>GGEERLETPSAKKLTDIGIRRIFSPEHDIFRKSVRKFFQEEVIPHHSEWEKAGEVSREVWEKAGKQGLLGVNIAEHLGGIGGDLYSAAIVWEEQAYSNCSGPGFSIHSGIVMSYITNHGSEEQIKHFIPQMTAGKCIGAIAMTEPGAGSDLQGIKTNAKKDGSDWILNGSKVFISNGSLSDVVIVVAVTNHEAPSPAHGISLFLVENGMKGFIKGRKLHKMGLKAQDTAELFFEDIRLPASALLGEENKGFYYIMKELPQERLLIADVAISASEFMFEETRNYVKQRKAFGKTVAHLQTVQHKLAELKTHICVTRAFVDNCLQLHEAKRLDSATACMAKYWASELQNSVAYDCVQLHGGWGYMWEYPIAKAYVDARVQPIYGGTNEIMKELIAREIVFDK[4x]

LCAD is a homotetramer containing one FAD per 43 kDa subunit with Glu291 as the catalytic base. LCAD substrate specificity overlaps those of VLCAD and MCAD, and in addition includes unsaturated and branched-chain substrates. Here we present the three-dimensional structure of human LCAD, revealing an unusually large substrate-binding cavity not previously reported in eucaryotic ACADs. The structural basis for the unique substrate binding cavity can be seen in the long E helix, where Pro132 is located in a position to cause unwinding of about two turns of the E helix, thus creating a large cavity.

Structures were obtained for wildtype LCAD complexed with and without acetoacetyl-CoA to 2.8 Å and 2.5 Å resolution, respectively. Although no substrates or inhibitors could be co-crystallized with wildtype crystals, the inhibitor acetoacetyl-CoA could be soaked into these crystals. Interestingly, only two monomers (Molecules A and B) of the tetramer have acetoacetyl-CoA bound, presumably due to the crystal packing. Binding of acetoacetyl-CoA to Molecules C and D would result in steric clashes between the adenine ring of FAD in Mol C and loop residues located between Glu151 and His156 of symmetry related Mol A, and between the FAD adenine of Mol D and the loop comprised of Glu105-His106-Leu107 of symmetry related Mol B. As in the structures of other acyl-CoA dehydrogenases, the carbonyl oxygen of the fatty acyl-CoA moiety of the substrate makes hydrogen bonds to the 2’-hydroxyl of the FAD ribityl chain (2.8 Å) and to the peptide backbone of (Gly412-N, 2.6 Å). New hydrogen bonding interactions contributing to significant CoA binding affinity are observed upon ligand binding. Arg424, situated at the entrance of the binding pocket, reorients from a position ~ 5.0 Å from the CoA phosphate into the active site, forming a hydrogen bond (3.3 Å) with the phosphate of the CoA. His228-Nε makes an H-bond with the phosphate of CoA. Having rotated approximately 125 degrees from its position in the unbound structure, the hydroxyl group of Tyr282 makes an H-bond with His228-ND1, so that the phenyl ring of Tyr282 stacks with the adenine ring of CoA. In the wild type structure, the chain starts at Glu34 (monomer A) or Leu36 (monomers B, C, and D). The C-terminal residue Lys430 is observed in all the monomers in the 2.8 Å structure of the wild type protein complexed with acetoacetyl-CoA, but not in the 2.5 Å wild type ligand-free and 2.0 Å (E291Q mutant) structures.> SEPPLHDFYCSRLLDLVFLLDGSSRLSEAEFEVLKAFVVDMMERLRVSQKWVRVAVVEYHDGSHAYIGLKDRKRPSELRRIASQVKYAGSQVASTSEVLKYTLFQIFSKIDRPEASRIALLLMASQEPQRMSRNFVRYVQGLKKKKVIVIPVGIGPHANLKQIRLIEKQAPENKAFVLSSVDELEQQRDEIVSYLCDLAPEA;> DCPSGWSSYEGNCYKFFQQKMNWADAERFCSEQ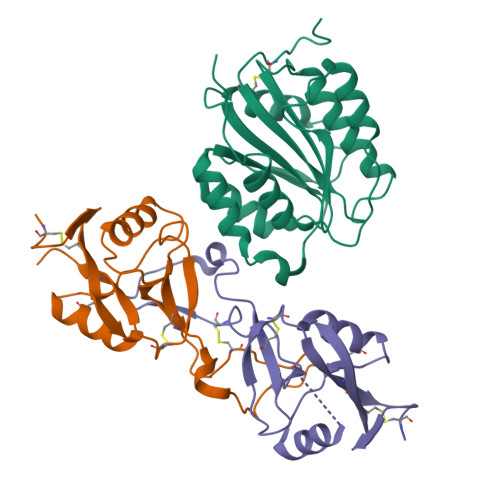AKGGHLVSIKIYSKEKDFVGDLVTKNIQSSDLYAWIGLRVENKEKQCSSEWSDGSSVSYENVVERTVKKCFALEKDLGFVLWINLYCAQKNPFVCKSPPP;> DCPPDWSSYEGHCYRFFKEWMHWDDAEEFCTEQQTGAHLVSFQSKEEADFVRSLTSEMLKGDVVWIGLSDVWNKCRFEWTDGMEFDYDDYYLIAEYECVASKPTNNKWWIIPCTRFKNFVCEFQA>[12x]MLRTMLKSKIHRATVTCADLHYVG;>[12x]XVTIDADLMDAADLLEGE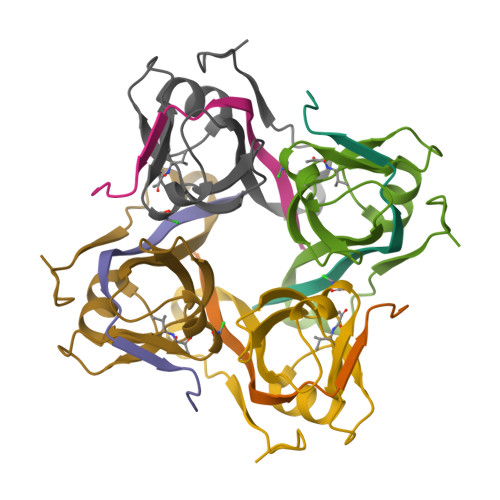QVTIVDIDNGARLVTYAITGERGSGVIGINGAAAHLVHPGDLVILIAYATMDDARARTYQPRIVFVDAYNKPIDMGHDPAFVPENAGELLDPRLGVGLEHHHHHH> 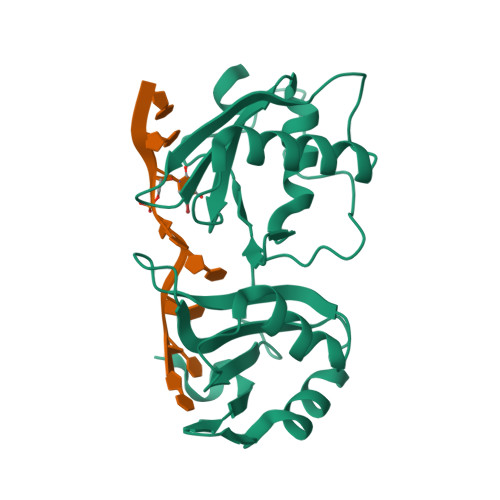GPLGSQMTRQARRLYVGNIPFGITEEAMMDFFNAQMRLGGLTQAPGNPVLAVQINQDKNFAFLEFRSVDETTQAMAFDGIIFQGQSLKIRRPHDYQPLPGMSENPSVYVPGVVSTVVPDSAHKLFIGGLPNYLNDDQVKELLTSFGPLKAFNLVKDSATGLSKDYAFCEYVDINVTDQAIAGLNGMQLGDKKLLVQRASVGAKN L-psicose | C6 H12 O6 | 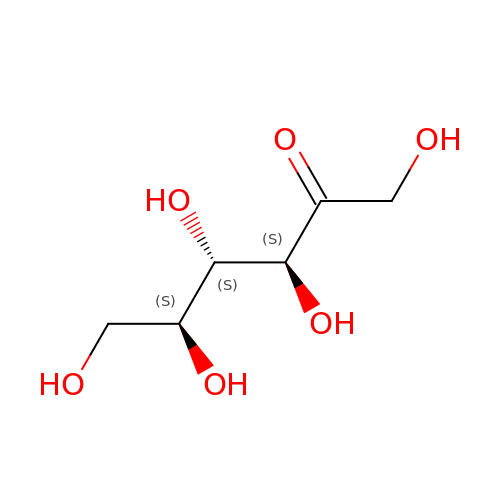BJHIKXHVCXFQLS-ZXEDONINSA-N>[2x]MFFTTPQPELSFDAMTIVGNLNKTNAKKLSDFMSTEPQIRLWDILQTKFKAKALQEKVYIEYDKVKADS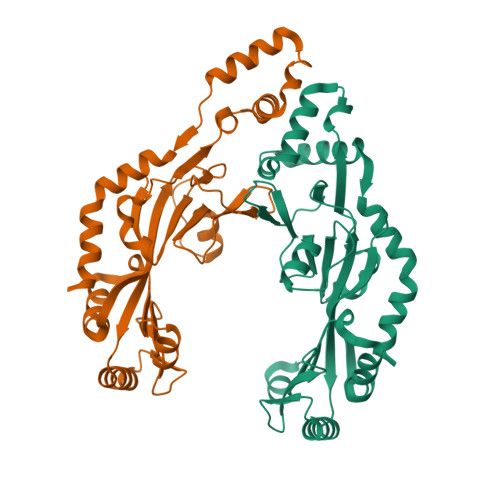WDRRNMRVEFNPNKLTHEEMLWLKQNIIDYMEDDGFTRLDLAFDFEDDLSDYYAMTDKAVKKTIFYGRNGKPETKYFGVRDSDRFIRIYNKKQERKDNADVEVMSEHLWRVEIELKRDMVDYWNDCFNDLHILKPDWSSLEKVKDQAMIYMLIHEESTWGKLERRTKNKYREMLKSISEIDLTDLMKLTLKENEKQLQKQIEFWQREFRFWE>SIGPVADLTISNGAVSPDGFSRQAILVNDVFPSPLITGNKGDRFQLNVIDNMTNHTMLKSTSIHWHGFFQHGTNWADGPAFVNQCPISTGHAFLYDFQVPDQAGTFWYHSHLSTQYCDGLRGPIVVYDPQDPHKSLYDVDDDSTVITLADWYHLAAKVGPAAPTADATLINGLGRSINTLNADLAVITVTKGKRYRFRLVSLSCDPNYTFSIDGHSLTVIEADGVNLKPQTVDSIQIFPAQRYSFVLNADQDVDNYWIRALPNSGTRNFDGGVNSAILRYEGAAPVEPTTSQTPSTQPLVESALTTLEGTAAPGNPTPGGVDLALNMAFGFAGGRFT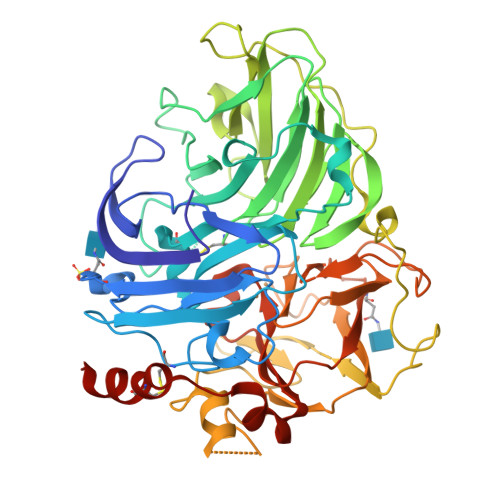INGASFTPPTVPVLLQILSGAQSAQDLLPSGSVYSLPANADIEISLPATSAAPGFPHPFHLHGHTFAVVRSAGSSTYNYANPVYRDVVNTGSPGDNVTIRFRTDNPGPWFLHCHIDFHLDAGFAVVMAEDTPDVAATNPVPQAWSDLCPTYDALSPDDQ[2x]>PPYTIVYFPVRGRAEAMRM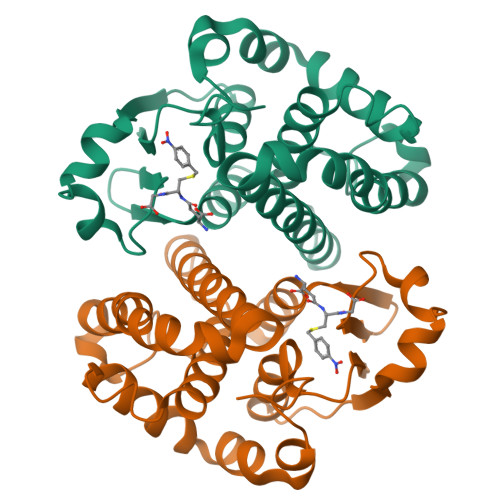LLADQGQSWKEEVVTIDTWMQGLLKPTCLYGQLPKFEDGDLTLYQSNAILRHLGRSLGLYGKNQREAAQMDMVNDGVEDLRGKYVTLIYTNYENGKNDYVKALPGHLKPFETLLSQNQGGKAFIVGDQISFADYNLLDLLLIHQVLAPGCLDNFPLLSAYVARLSARPKIKAFLSSPEHVNRPINGNGKQ[2x]> MTATVGRWMGPAEYQQMLDTGTVVQSSTGTTHV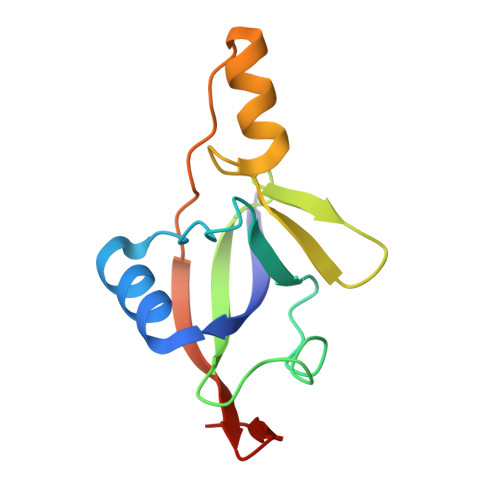AYPADIDAFGKQAKNGAMYVEFDVPEKSLVPTNEGWAKIVGPDSIEGRLAKRKGLPVPEMPTAENITVRGEKINGEVEAKC>GPMSEAVKNLVNNDLADVMFNRHSVRQFDPNVKIGRDELQKMIAEAATAPSACNLQSWHFVVVDTPEAKAKFKQAVMKFNYPQVDSASAIVFIAGDTQSHYVYRDVWNKVYEDGNITKERLDQILGTFLPLYE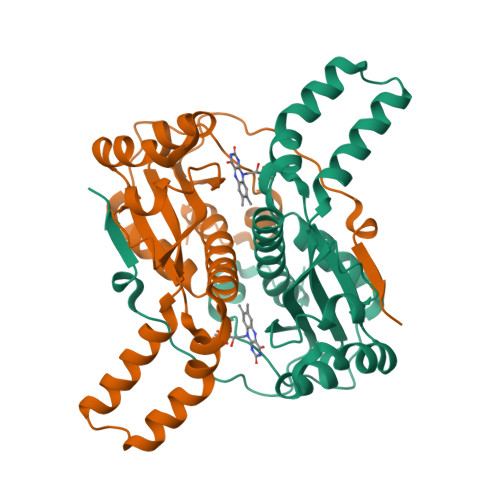NATPDFLKFDATIDCSVVGMQLLLVARAHGYDANAFSGIDFEKMIPTLGLDPKRYVPVMGIAIGKAAQEPLHTTRYDAKTQTDFLA[4x]>KSPSAQELKEQGNRLFVGRKYPEAAACYGRAITRNPLVAVYYTNRALCYLKMQQHEQALADCRRALELDGQSVKAHFFLGQCQLEMESYDEAIANLQRAYSLAKEQRLNFGDDIPSALRIAKKKRWNS[2x];>[2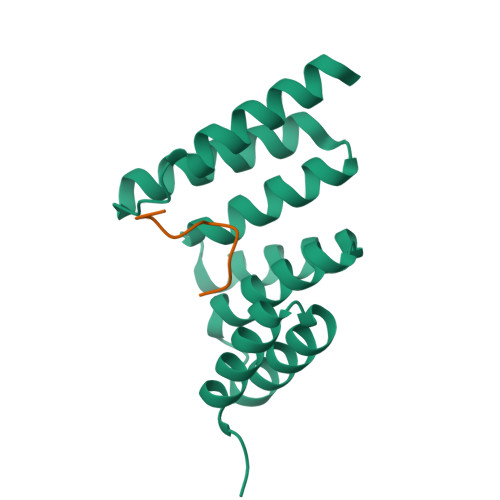x]SSTGSIDMVD> MWLFFGITGLLTAALSGHPSPAPPDQLNTSSAESELWEPGERLPVRLTNGSSSCSGTVEVRLEASWEPACGALWDSRAAEAVCRALGCGGAEAASQLAPPTPELPPPPAAGNTSVAANATLAGAPALLCSGAEWRLCEVVEHACRSDGRRARVTCAENRALRLVDGGGACAGRVEMLEHGEWGSVCDDTWDLEDAHVVCRQLGCGWAVQALPGLHFTPGRGPIHRDQVNCSGAEAYLWDCPGLPGQHYCGHKEDAGVVCSEHQSWRLTGGADRCEGQVEVHFRGVWNTVCDSEWYPSEAKVLCQSLGCGTAVERPKGLPHSLSGRMYYSCNGEELTLSNCSWRFNNSNLCSQSLAARVLCSASRGHHHHHH

CD6 is a transmembrane protein with an extracellular region containing three scavenger receptor cysteine rich (SRCR) domains. The membrane proximal domain of CD6 binds the N-terminal immunoglobulin superfamily (IgSF) domain of another cell surface receptor, CD166, which also engages in homophilic interactions. CD6 expression is mainly restricted to T cells, and the interaction between CD6 and CD166 regulates T-cell activation. We have solved the X-ray crystal structures of the three SRCR domains of CD6 and two N-terminal domains of CD166.

The X-ray structure of CD6 is the first structure for a protein containing consecutive SRCR domains. The structure reveals a nonlinear organization of consecutive SRCR domains of CD6. Despite the interdomain interactions not being conserved, the orientations of each domain relative to its adjacent domain are very similar, both burying approximately 270 Å2. A consequence of this orientation at the interfaces between individual SRCR domains is a nonlinear consecutive domain structure, resulting in the three domains spanning 78.1 Å, a shorter distance than if the domains were in a linear arrangement. There is a disordered region in CD6 domain 1 in a similar position to a flexible loop in CD5 domain 1 (Garza-Garcia et al., 2008). In the recombinant protein, we observed electron density for GlcNAc attached to residue N229 in the second domain. There was no observable electron density for the other potential glycosylation sites in CD6. Using our structure of CD6 and previous mutagenesis data (Bodian et al., 1997; Skonier et al., 1997), we carried out a more extensive mutagenesis study on CD6 domain 3 to define the residues critical for CD166 binding. These data were mapped onto the structure, clearly identifying and defining the boundaries of the surface of CD6 that interacts with CD166. The CD6 surface features a stripe of negative charge flanked with positive charge, and the CD166 surface features a complementary positively charged stripe flanked by negative charge. Homozygotes for two of these SNPs (R225W and A257V) in domain 2 have been associated with susceptibility to multiple sclerosis (Swaminathan et al., 2013). These two residues are buried within the domain and may disrupt the domain structure and stability of the molecule, explaining the correlation between reduced expression and susceptibility to multiple sclerosis.> GSMASSSSSERWIDGLQFSSLLWPPPRDPQQHKDQVVAYVEYFGQFTSEQFPDDIAELVRHQYPSTEKRLLDDVLAMFVLHHPEHGHAVILPIISCLIDGSLVYSKEAHPFASFISLVCPSSENDYSEQWALACGEILRILTHYNRPIYKTEQQNGDTERNCLSKATTSGSPTSEPKAGSPTQHERKPLRPLSPWISDILLAAPLGIRSDYFRWCSGVMGKYAAGELKPPTIASRGSGKHPQLMPSTPRWAVANGAGVILSVCDDEVARYETATLTAVAVPALLLPPPTTSLDEHLVAGLPALEPYARLFHRYYAIATPSATQRLLLGLLEAPPSWAPDALDAAVQLVELLR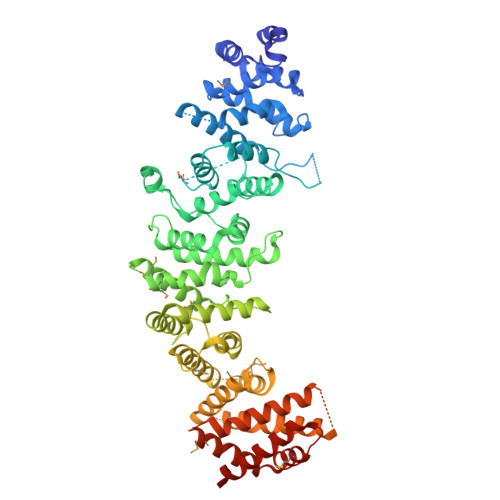AAEDYASGVRLPRNWMHLHFLRAIGIAMSMRAGVAADAAAALLFRILSQPALLFPPLSQVEGVEIQHAPIGGYSSNYRKQIEVPAAEATIEATAQGIASMLCAHGPEVEWRICTIWEAAYGLIPLNSSAVDLPEIIVATPLQPPILSWNLYIPLLKVLEYLPRGSPSEACLMKIFVATVETILSRTFPPESSRELTRKARSSFTTRSATKNLAMSELRAMVHALFLESCAGVELASRLLFVVLTVCVSHEAQSSGSKRPRSEYASTTENIEANQPVSNNQTANRKSRNVKGQGPVAAFDSYVLAAVCALACEVQLYPMISGGGNFSNSAVAGTITKPVKINGSSKEYGAGIDSAISHTRRILAILEALFSLKPSSVGTPWSYSSSEIVAAAMVAAHISELFRRSKALTHALSGLMRCKWDKEIHKRASSLYNLIDVHSKVVASIVDKAEPLEAYLKNTPVQKD> IPAWASGN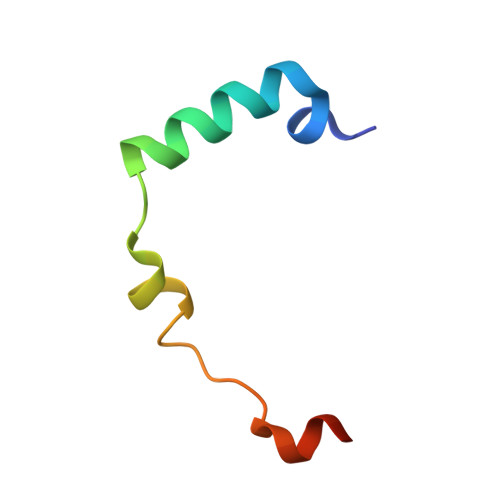LLTQAIRQQYYKPIDVDRMYGTIDSPKLEELFNKS> ESRTSAPSGCLTVGSDGTYSTIGDALDALGSSTSSACIYVASGTYEEQLTIDYAGNLTLYGETTDTSTYKDNVVTITHTISSPDAGSLDKSATVNVVSDGFSMYNINVENGYGEGAQAVALVGNADQLGFYGCQFSGYQDTLYVKAGTQYYSNCMIEGAVDYIFGDASVWFGECDIVSN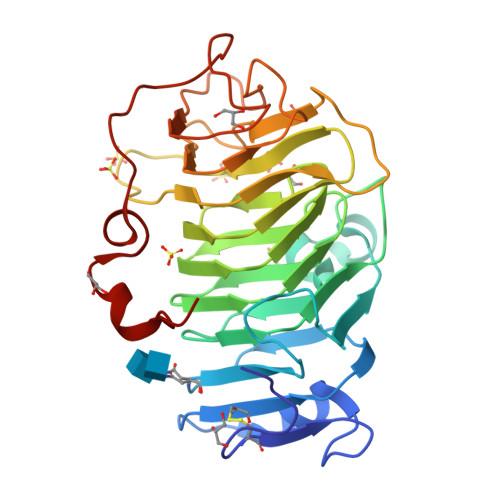GAGAITASSRETSSDSGWYAIDNCNIKAASGVSLTEEVYLGRPWRVLARVIYQNSVLSDIINPKGWTTMADGATPLYYEYNNSGAGSDTSDREYETSISAAVDKTTVLGETWGDWIDRSY>MEEPEEPADSGQSLVPVYIYSPEYVSMCDSLAKIPKRASMVHSLIEAYALHKQMRIVKPKVASMEEMATFHTDAYLQHLQKVSQEGDDDHPDSIEYGLGYDCPATEGIFDYAAAIGGATITAAQCLIDGMCKVAINWSGGWHHAKKDEASGFCYLNDAVLGILRLRRKFERILYVNLDLHHGDGVEDAFSFTSKVMTVSLHKFSPGFFPGTGDVSDVGLGKGRYYSVNVPIQDGIQDEKYYQICESVLKEVYQAFNPKAVVLQLGADTIAGDPMCSFNMTPVGIGKCLKYILQWQLATLILGGGGFNLANTARCWTYLTGVILGKTLSSEIPDHEFFTAYGPDYVLEITPSCRPDRNEPHRIQQILNYIKGNLKHV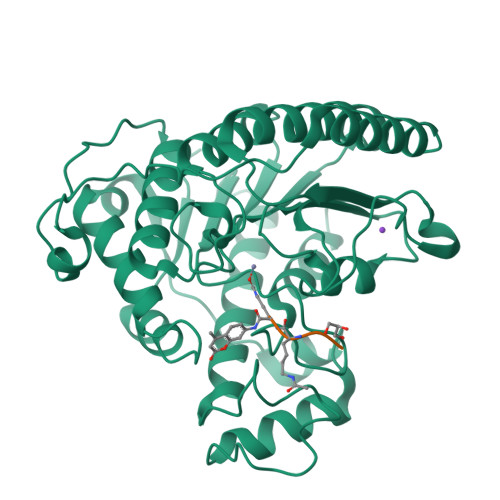VIEGRGSHHHHHH[2x]> MNTKYNKEFLLYLAGFVDGDGSIIAQIKPNQSSKFKHRLSLTFQVTQKTQRRWFLDKLVDEIGVGYVRDSGSVSNYILSEIKPLHNFLTQL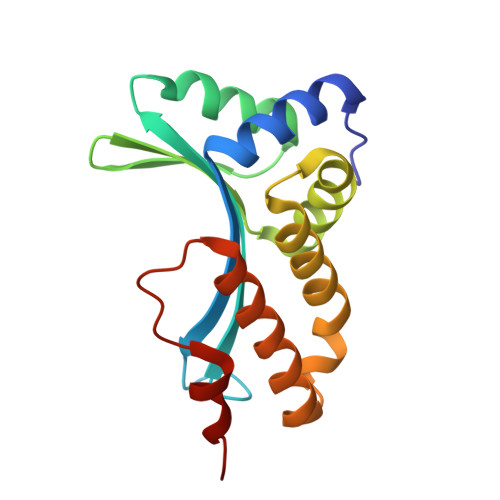QPFLKLKQKQANLVLKIIEQLPSAKESPDKFLEVCTWVDQIAALNDSKTRKTTSETVRAVLD>[2x]GNSFVGLRVVAKWSSNGY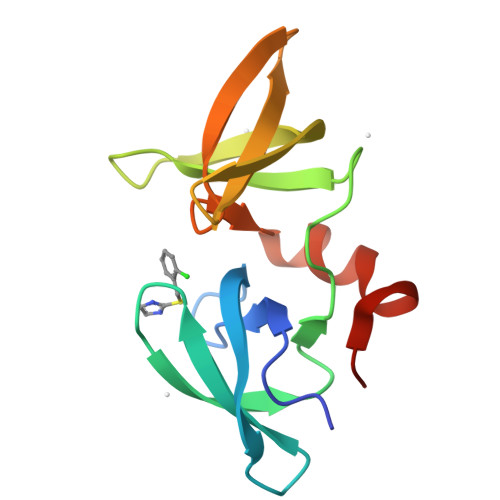FYSGKITRDVGAGKYKLLFDDGYECDVLGKDILLCDPIPLDTEVTALSEDEYFSAGVVKGHRKESGELYYSIEKEGQRKWYKRMAVILSLEQGNRLREQYGLGPYE>MGQYKKLWYLLFAVLAVCFTILGYMGSEVYKKAPPYPEQVVSASGKVLMAKDDILAGQSAWQTTGGMEVGSVLGHGAYQAPDWTADWLHRELSAWLDLTAQQTYGKKFDEVSPEEQAVLKTRLADEYRNQSRIKEDGSVVISDTRVKAIESILPYYHGVYGDDPALQTTREHFAMKNNTLPSQEAREKLFDFFFWTSWSASTNRPDETFTYTNNWPHEPLINNVPTTENYMWSFTSVVLLLMGIGLLMWGYSFLTKHEEVEVPTEDPISKVQLTPSQKALGKYVFLTVALFVVQVLLGGLTAHYTVEGQGFYGIDEALGFEMSDWFPYALTRTWHIQSAIFWIATGFLTAGLFLAPIVNGGKDPKFQRAGVNFLYIALFIVVGGSYAGNFFALTHILPPEFNFWFGHQGYEYLDLGRFWQLLLMVGLLLWLFLMLRCTVSAFKEKGVDKNLLAIFVASMVGVGVFYAPGLFYGEKSPIAVMEYWRWWVVHLWVEGFFEVFATAAFAFVFYNMGFVRRSTATASTLAAAAIFMLGGVPGTLHHLYFSGSTSASMAIGACFSALEVVPLVLLGREAYEHWSYQHLSEWAKRLRWPLMCFVAVAFWNMIGAGVFGFLINPPISLFYIQGLNTSAVHAHAALFGVYGFLALGFVLLVARYLKPNVQFDDKLMTWGFWLLNGGLVGMIAISLLPVGVIQAYASITHGLWYARSEEFLQMEILDTLRWVRTAADLIFIGGAICVAIQATKIVFGRDK[2x]

A quinol-dependent nitric oxide reductase (qNOR) plays a critical role in the survival of the bacterium in the human host by combatting the host’s immune response. qNORs belong to the broader family of nitric oxide reductases (NORs). NORs are largely found as the essential component of anaerobic nitrate respiration, also known as denitrification, in the bacterial cytoplasmic membrane and catalyse the reduction of nitric oxide (NO) to nitrous oxide (N2O). Whilst cNORs are pre­dominantly found in denitrifying organisms as a respiratory enzyme, qNORs are also found in several pathogenic bacteria, including the Gram-negative, human-pathogenic bacterium N. meningitidis, as an enzyme that is responsible for the detoxification of NO produced by the host. High-resolution structure determination of N. meningitidis qNOR (NmqNOR) is of importance to provide a framework for developing a knowledge-based strategy for the design of new antibacterial agents, as well as to help to understand the chemistry of NO reduction, 2NO + 2 H+ + 2e− → N2O + H2O, at the heme and nonheme iron (FeB) binuclear centre.

For the final 3D reconstruction with C2 symmetry imposed, a final global resolution of 3.06 Å was achieved, as judged by the ‘gold standard’ FSC = 0.143. 3, FeB and their associated ligands could be modelled with confidence. The coordination of the active site in the absence of zinc was observed by cryo-EM, which interestingly showed that FeB was ligated by four ligands: the three conserved histidine ligands (His490, His541 and His542) and Glu494 [Fig. 4(a)]. The dimeric structure of NmqNOR is largely maintained by TMII, similar to as in AxqNOR. Along TMII, structural analysis using PyMOL (version 1.8; Schrödinger) revealed a cavity that bridges the dimeric interface connecting the two monomers [Supplementary Figs. S5(b) and S5(c)]. At the end of this putative water channel lie Glu498 and Asn604, which are ligated and may serve as a ‘junction’ that is responsible for controlling the proton before entering the active site; our previous study shows that mutation of Glu498 reduces the activity of this enzyme. For the crystal structure, the crystal was grown under zinc-containing conditions, which led to the observation of three zinc-binding sites, with the Zn2 binding site affecting the conformation of Glu494. However, a native dimeric structure was observed in the cryo-EM structure as the data were collected without any additional buffer components; in this structure Glu494 was ligated to FeB, which we believe is the natural position for Glu494 [Fig. 6(a)].>[2x]MELYVNFELPPEAEEELRKYFKIVRGGDLGNVEAALVSRITAEELAKMPRLKFIQVVTAGLD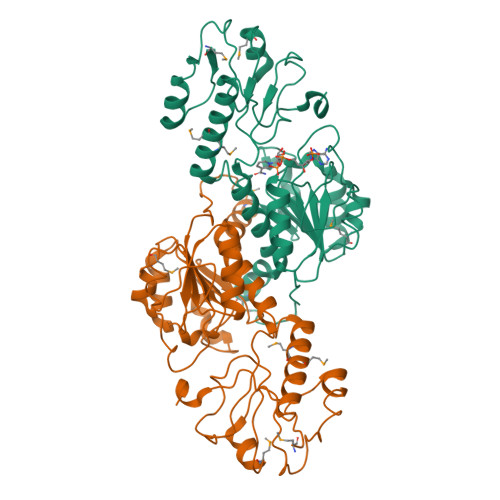HLPWESIPPHVTVAGNAGSNADAVAEFALALLLAPYKRIIQYGEKMKRGDYGRDVEIPLIQGEKVAVLGLGEIGTRVGKILAALGAQVRGFSRTPKEGPWRFTNSLEEALREARAAVCALPLNKHTRGLVKYQHLALMAEDAVFVNVGRAEVLDRDGVLRILKERPQFIFASDVWWGRNDFAKDAEFFSLPNVVATPWVAGGYGNERVWRQMVMEAVRNLITYATGGRPRNIAKREDYIGS2,3,7,8-tetrahydroxychromeno[5,4,3-cde]chromene-5,10-dione | C14 H6 O8 | 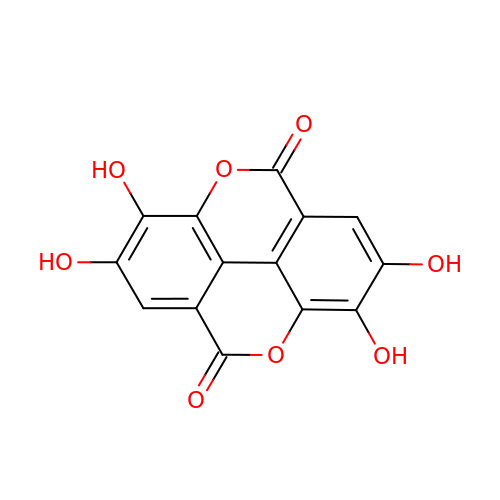AFSDNFLWKVMVRB-UHFFFAOYSA-N>[4x]ATQGVFTLPANTRFGVTAFANSSGTQTVNVLVNNETAAT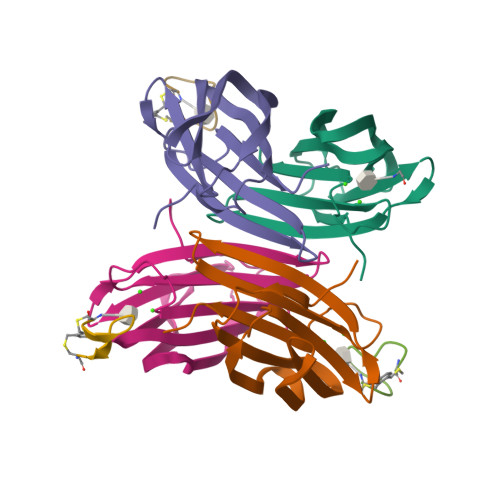FSGQSTNNAVIGTQVLNSGSSGKVQVQVSVNGRPSDLVSAQVILTNELNFALVGSEDGTDNDYNDAVVVINWPLG;>[3x]CWWKKKKKWWCX;> GGGGG5'-O-[(S)-amino(hydroxy)phosphoryl]adenosine 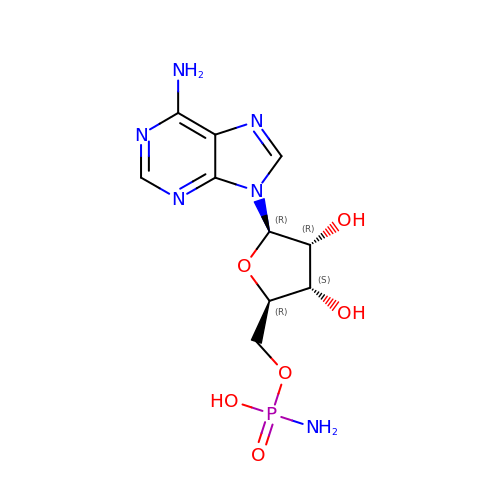| C10 H15 N6 O6 P | LDEMREUBLBGZBO-KQYNXXCUSA-N>[3x]MGSSHHHHHHENLYFQGSMEQAIINDER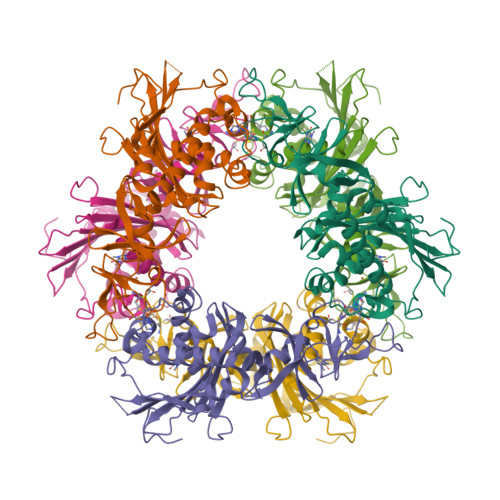EYLRHFWHPVCTVTELEKAHPSSLGPLAVKLLNEQLVVAKLGDEYVAMRDRCAHRSAKLSLGTVSGNRLQCPYHGWQYDTHGACQLVPACPNSPIPNKAKVDRFDCEERYGLIWIRLDSSFDCTEIPYFSAANDPRLRIVIQEPYWWDATAERRWENFTDFSHFAFIHPGTLFDPNNAEPPIVPMDRFNGQFRFVYDTPEDMAVPNQAPIGSFSYTCSMPFAINLEVSKYSSSSLHVLFNVSCPVDSHTTKNFLIFAREQSDDSDYLHIAFQDLVLAEDKPVIESQWPKDAPADEVSVVADKVSIQYRKWLRELKEAHKEGSQAFRSALLDPVIESDRSYI>SEAAKKALNDYIWGLQYDKLNILTHQGEKLKNHSSREAFHRPGEYVVIEKKKQSISNATSKLSVSSANDDRIFPGALLKADQSLLENLPTLIPVNRGKTTISVNLPGLKNGESNLTVENPSNSTVRTAVNNLVEKWIQKYSKTHAVPARMQYESISAQSMSQLQAKFGADFSKVGAPLNVDFSSVHKGEKQVFIANFRQVYYTASVDSPNSPSALFGSGITPTDLINRGVNSKTPPVYVSNVSYGRAMYVKFETTSKSTKVQAAIDAVVKGAKLKAGTEYENILKNTKICAVVLGGNPGEASKVCTGNIDTLKDLIQKGSNFSAQSPAVPISYTTSF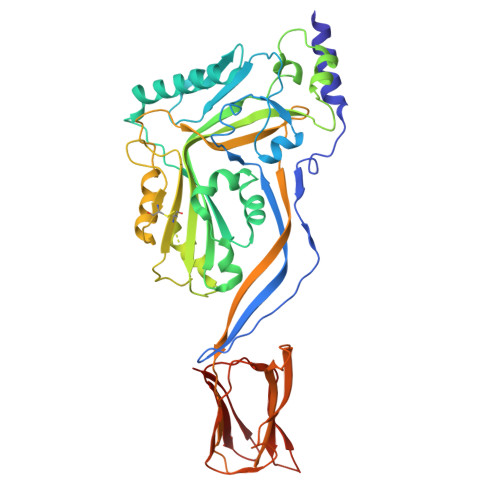VKDNSIATIQNNTDYIETKVTSYKDGALTLNHDGAFVARFYVYWEELGHDADGYETIRSRSWSGNGYNRGAHYSTTLRFKGNVRNIRVKVLGATGLAWEPWRLIYSKNDLPLVPQRNISTWGTTLHPQFEDKVV[2x]> APLLESQRSNSEEKANFCSTHNDEVYARFRLQMRVGVRHSPLYTPSNMCMLDIEDSVEDIEESTEKEYASTATGEAAGVNVSVALVGEGVSIPFSYIGLGFNPSLEDSYLYVNVSSRAPWVKQTSDLSANGGWGIKQVLEKELLAIQIGCDNQKFPEEPTTTPPSPVTTTLSSTTPDLNEENTENTPTTTGASVDRKRNPADIDFSL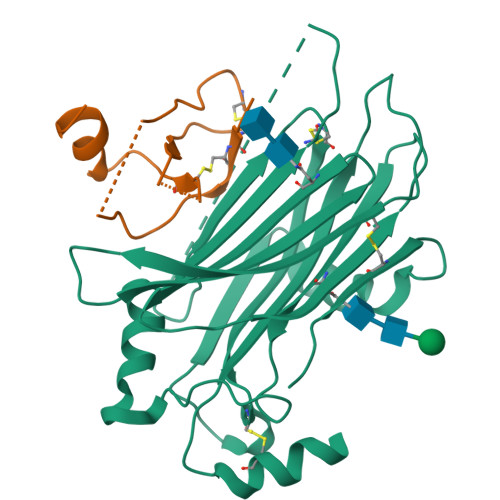LVDPRCVTSVDLHVELRDACIDYKQESPLSLKGKYGDGELVKKEIKDVGKNHNMCSLNLNPGNENLYFQ;> SLAADTPTACCFSYTSRQIPQNFIADYFETSSQCSKPGVIFLTKRSRQVCADPSEEWVQKYVSDLELSAHHHHHH>[2x]GPLGSPEFGYWITCCPTCDVDINTWVPFYSTELN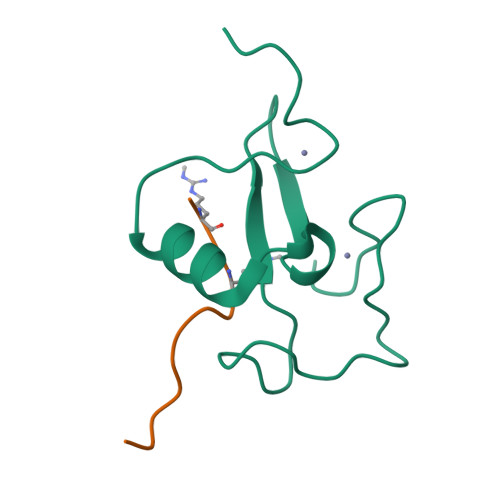KPAMIYCSHGDGHWVHAQCMDLEERTLIHLSEGSNKYYCNEHVQIARA;>[2x]ARTKQTARKAAG> KDMFN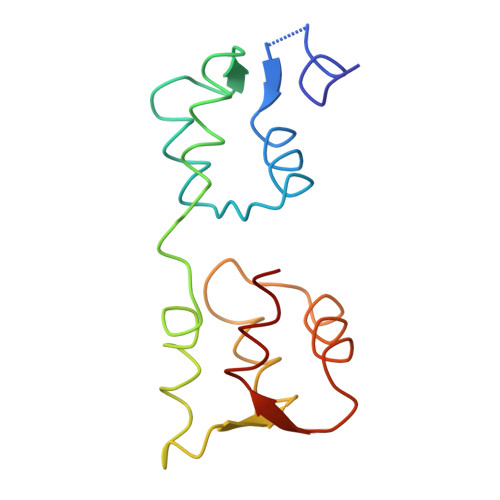TKSSNGKLRIEDASHNARKLGLAPSSTDEKKIRDLYGDSLTYEQYLEYLTMCVHDRDNMEELIKMFSHFDNNSSGFLTKNQMKNILTTWGDALTEQEANDALNAFSSEDRINYKLFCEDILS>[10x]GSHMASKGNIEVLNLVTGPDSITTIELYLNTRMGQNDESKDNYGYSEKVTVANSSDQDKPTSGEIPTYSTARINLPMLNEDLTCNTLTMWEAVSVKTEVVGVSSLVNVHMATKRMYDDKGIGFPVEGMNFHMFAVGGEPLELQFLTGNYRTDYSANDK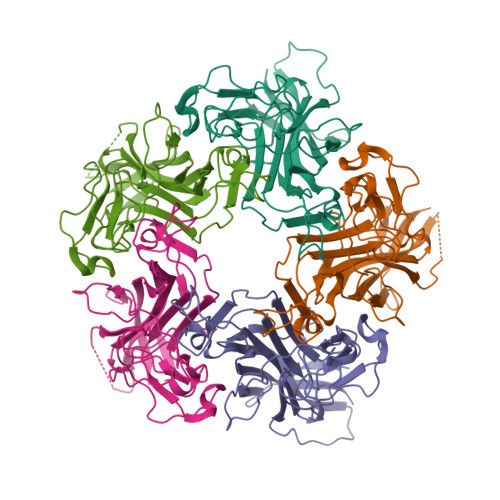LVVPPIKHQSTQGLNPHYKQKLTKDGAFPVECWCPDPSKNENTRYYGSYTGGQSTPPVLQFTNTVTTVLLDENGVGPLCKGDGLYVSCCDIVGFLVGKDGDMQYRGLPRYFNILLRKRTVRN>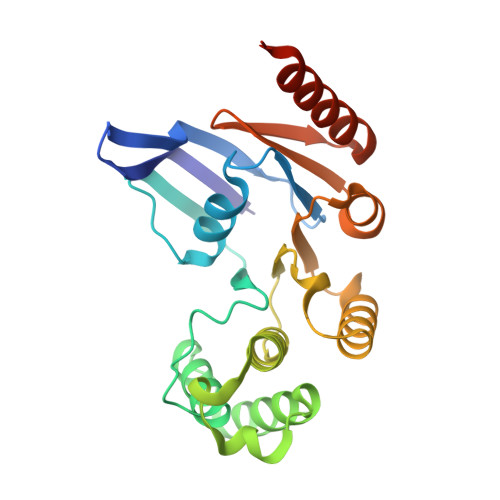 MIELRNLTKWYPTPHGRRYVFRNLNFRFPDDVSIGLIGRNGAGKSTLMRLLGGIEAPNEGEVVTDVSISWPVGLSGGFQGSLTARENVKFVCRIYGTSHEDMLRKVRFVEEFAEIGEHFDLPMKTYSSGMRSRVAFGLSMAFDFDYYLIDEAMAVGDAQFRAKSRAVFDSRVGQANMILVSHNMNDIKEYCDVVVLVDQGQATLYEDVEAGIAAYQGSLKKAAAKPDYKDDDDK> MDQSVSNVDKSSAFEYNKMIGHGINMGNALEAPVEGSWGVYIEDEYFKI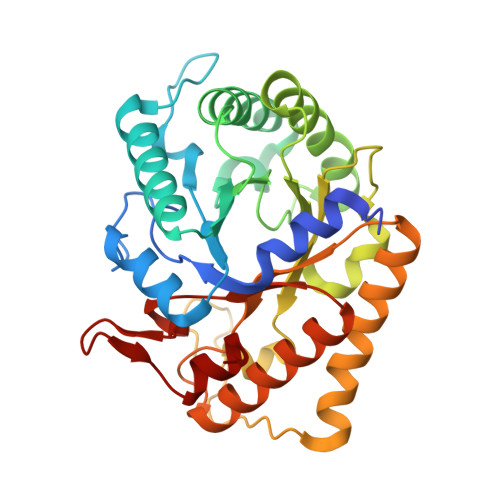IKERGFDSVRIPIRWSAHISEKYPYEIDKFFLDRVKHVVDVALKNDLVVIINCHHFEELYQAPDKYGPVLVEIWKQVAQAFKDYPDKLFFEIFNEPAQNLTPTKWNELYPKVLGEIRKTNPSRIVIIDVPNWSNYSYVRELKLVDDKNIIVSFHYYEPFNFTHQGAEWVSPTLPIGVKWEGKDWEVEQIRNHFKYVSEWAKKNNVPIFLGEFGAYSKADMESRVKWTKTVRRIAEEFGFSLAYWEFCAGFGLYDRWTKTWIEPLTTSALGK> GPAFEFAVAMMKRNSSTVKTEYGEFTMLGIYDRWAVLPRHAKPGPTILMNDQEVGVLDAKELVDKDGTNLELTLLKLNRNEKFRDIR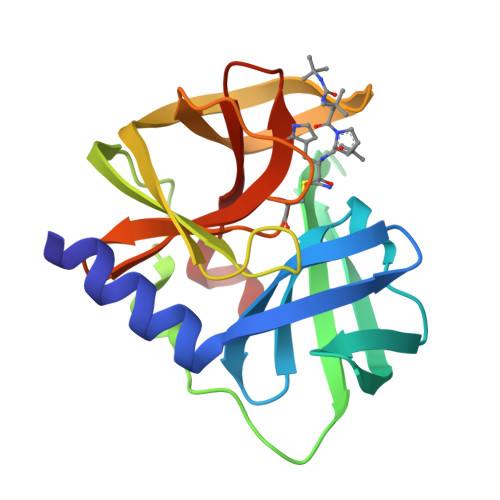GFLAKEEVEVNEAVLAINTSKFPNMYIPVGQVTEYGFLNLGGTPTKRMLMYNFPTRAGQCGGVLMSTGKVLGIHVGGNGHQGFSAALLKHYFN>[2x]MVPSYDSFDYEDYPAALPNHKPKGTFKDYVRDRA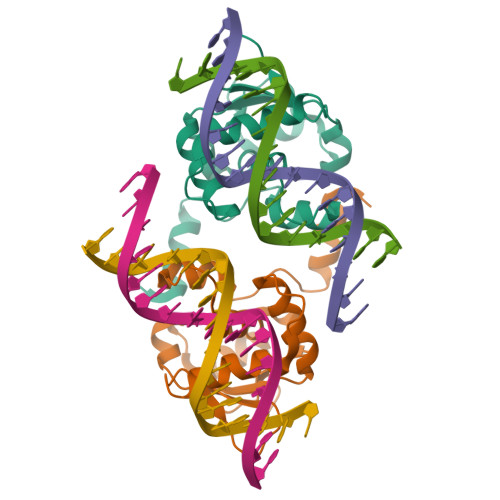DLNKDKPVIPAAALAGYTGSGPIQLWQFLLELLTDKSCQSFISWTGDGWEFKLSDPDEVARRWGKRKNKPKMNYEKLSRGLRYYYDKNIIHKTAGKRYVYRFVCDLQSLLGYTPEELHAMLDVKPDADE> MANTSRTRQALMAIAVSVLAAGVTTLGVAHADNGDAVAAAAEMPQAVEDFSYPGAAKIQAETGAILKRGNGHMLMTSCDGSEDI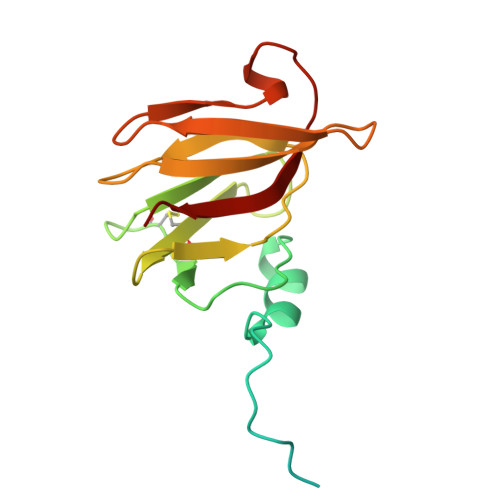QVMSRTGQKDFCFNVMAKPAYLTLEVPQAYGIWTSADPVKTTIKDTDGTATVINAPANDFTGYGEAGSTGEPTTLIELRVAG> RKTPEELLRQNQRALNRAMRELDRERQKLETQEKKIIADIKKMAKQGQMDAVRIMAKDLVRTRRYVRKFVLMRANIQAVSLKIQTLKSNNSMAQAMKGVTKAMGTMNR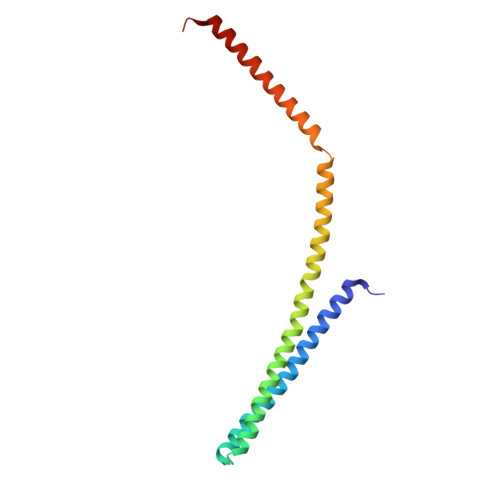QLKLPQIQKIMMEFERQAEIMDMKEEMMNDAIDDAMGDE> IVGGRRARPHAWPFMVSLQLRGGHFCGAT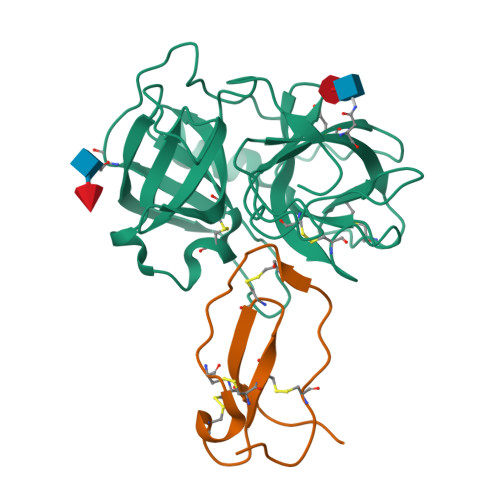LIAPNFVMSAAHCVANVNVRAVRVVLGAHNLSRREPTRQVFAVQRIFENGYDPVNLLNDIVILQLNGSATINANVQVAQLPAQGRRLGNGVQCLAMGWGLLGRNRGIASVLQELNVTVVTSLCRRSNVCTLVRGRQAGVCFGDSGSPLVCNGLIHGIASFVRGGCASGLYPDAFAPVAQFVNWIDSIIQ;> RRKPGKCPVTYGQCLMLNPPNFCEMDGQCKRDLKCCMGMCGKSCVSPVKA>GGGGGPGELGKPVRLPKEMSDEMKKAVDDGWTKNAFNQYVSDLISVHRTLPDPRDAWCKDEARYLTNLPKTDVIICFHNEAWTVLLRTVHSVLDRSPEHLIGKIILVDDYSDMPHLKRQLEDYFAAYPKVQIIRGQKREGLIRARILGANHAKSPVLTYLDSHCECTEGWLEPLLDRIARNSTTVVCPVIDVISDETLEYHYRDSGGVNVGGFDWNLQFSWHPVPERERKRHNSTAEPVYSPTMAGGLFSIDREFFDRLGTYDSGFDIWGGENLELSFKTWMCGGTLEIVPCSHVGHI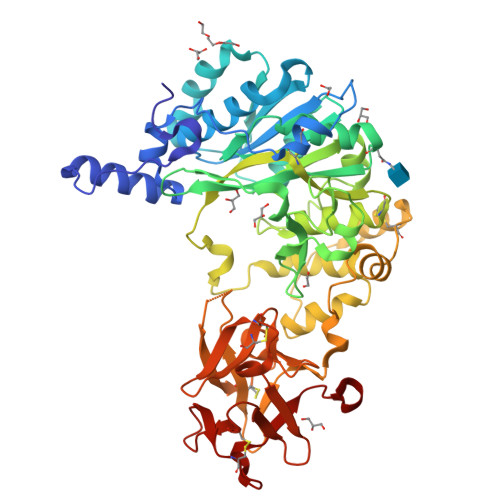FRKRSPYKWRSGVNVLKKNSVRLAEVWMDEYSQYYYHRIGNDKGDWGDVSDRRKLRNDLKCKSFKWYLDNIYPELFIPGDSVAHGEIANVPNGMCLDAKEKSEEETPVSIYECHGQGGNQYWMLSKAGEIRRDDSCLDYAGKDVTLFGCHGGKGNQFWTYRENTKQLHHGTSGKCLAISESKDKLLMEECSASLSRQQWTLENYDSSKL[2x]> MDDLVFAGNKA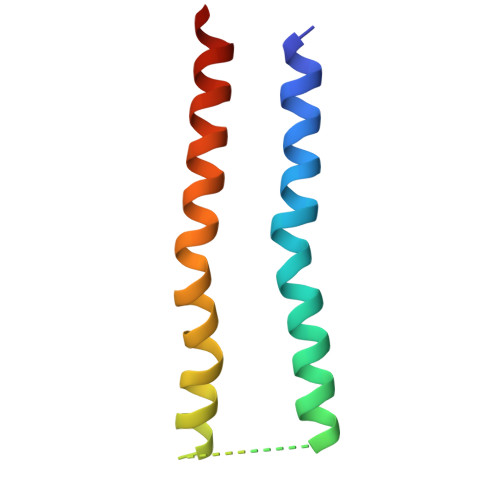LYLVLILSGWPTIVATIIGLLVGLFQTVTQLQEQTLPFGIKLLGVCLCLFLLSGWYGEVLLSYGRQVIFLALAKG> MSRVQMDTEEVREFVGHLERFKELLREEVNS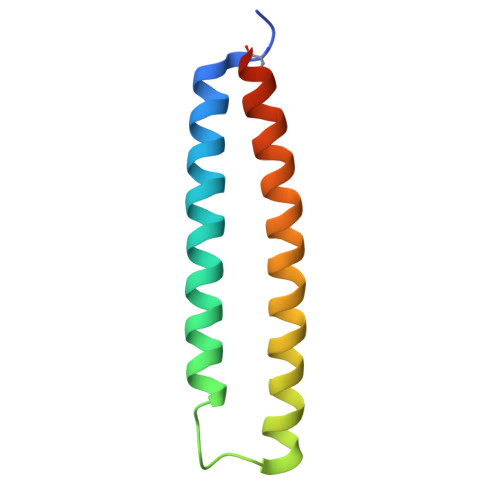LSNHFHNLESWRDARRDKFSEVLDNLKSTFNEFDEAAQEQIAWLKERIRVLEEDY>GPLGSETITVPTPIKQIFSDDAFAETIKDNLKKKSVTDAVTQNELNSIDQIIANNSDIKSVQGIQYLPNVTKLFLNGNKLTDIKPLANLKNLGWLFLDENKVKDLSSLKDLKKLKSLSLEHNGISDINGLVHLPQLESLYLGNNKITDITVLSRLTKLDTLSLEDNQISDIVPLAGLTKLQNLYLSKNHISDLRALAGLKNLDVLELFSQECLNKPINHQSNLVVPNTVKNTDGSLVTPEIISDDGDYEKPNVKWHLPEFTNEVSFIFYQPVTIGKAKARFHGRVTQPLKEVYTVSYDVDGTVIKTKVEAGTRITAPKPPTKQGYVFKGWYTEKNGGHEWNFNTDYMSGNDFTLYAVFKAET[3x]

InlB, an invasion protein from the facultative intracellular pathogen Listeria monocytogenes, is a multi-domain protein that binds and activates the human receptor tyrosine kinase MET. The N-terminal internalin domain (amino acids 36–321; InlB321) is characterized by a central leucine-rich repeat (LRR) region that binds to the first Ig-like IPT domain of MET with high affinity. The LRR region is flanked N-terminally by a helical cap and C-terminally by an Ig-like inter-repeat (IR) region. The B repeat folds into a compact domain resembling a β-grasp fold.

Intriguingly, wild-type InlB392 was a much more problematic crystallization target than the InlB392_T332E variant. Crystals only grew in condition E6 of a MORPHEUS screen stored beyond its ‘use by’ date. At 4°C we obtained thin rod-shaped crystals with a cross-section of about 10 × 10 µm and a length of 80–100 µm. The best crystal diffracted to 3.3 Å resolution. The packing of InlB392_T332E crystal form I is closely related to that of InlB392_wt and the surroundings of all three molecules in the wild-type structure are similar. In a way, the packing of InlB392_wt can be viewed as a slightly distorted version of InlB392_T332E crystal form I with a tripled b axis.> MTTVLVTGGAGFIATHTDIELLNKGYDVISVDNYGNSSPVALERVEQITGKPVKRYDGDVRDEALMERVFAENNIDWVIHFAGLKAVGESVAKPIEYYDNNLYSTLVLLKVMKKHNVKKIIFSSSATVYGTPKELPITEETPTGGTTNPYGTSKLFQEQILRDVHVADPSWT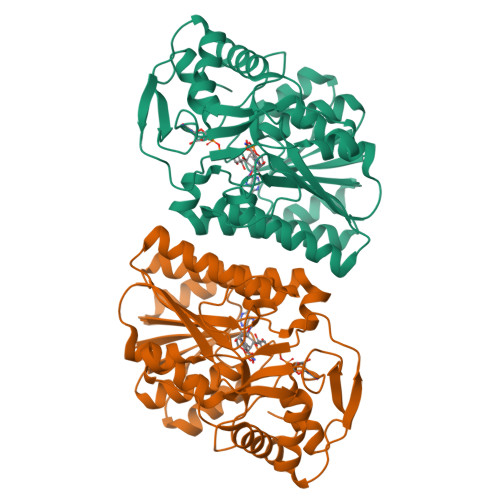IVLLRYFNPVGAHESGLLGEDPKGIPANLTPYVAKVAVGELKEVQVYGDDYDTPDGTGVRDYIHVVDLAKGHVAVIDHIDKEGVFVYNLGTGHGYSVLEVIKAYEKAAGHPIPYAIKPRRPGDIAACYADASKAEKELGWKAELTIDDMAASSLNWQTKNPNGFRDAE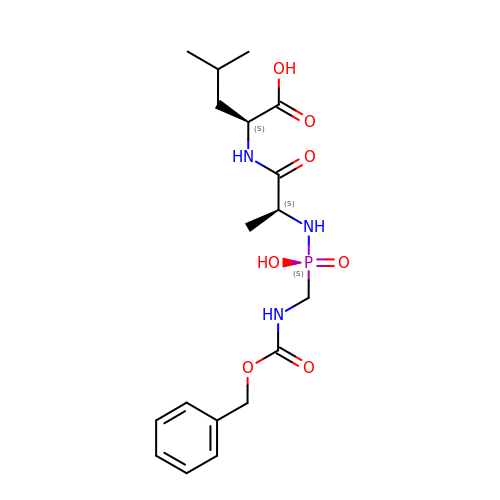N-[(S)-({[(benzyloxy)carbonyl]amino}methyl)(hydroxy)phosphoryl]-L-alanyl-L-leucine | C18 H28 N3 O7 P | RFIATXCLWWIOFV-ZFWWWQNUSA-N> MFTRFVTQPTLLTQTQRALFSALTKKQKMEVTLRTPYKEYLANFDGFSRITAKTNEASLVIQNKTPASLYVLPPGPLKIRFTSEVKNVSGDFLHTGGWVIVHADNTCEINVMDLFDRKEVRADQFEKGNIQDLDTLAGKYAAKSRKSTVRLFT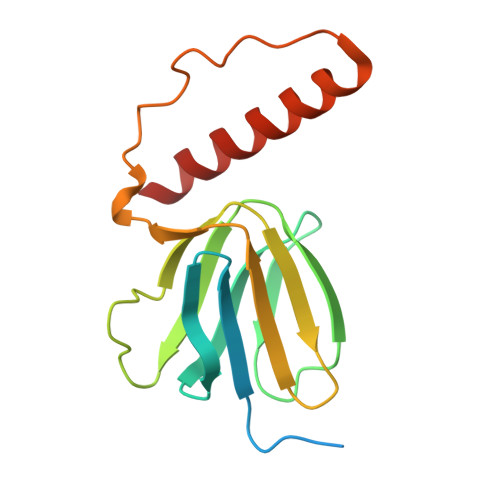KATTQ>GVTELSDAQKKQLKEQQEMQQMYDMIMQHKRAMQDMQLLWEKAVQQHQHGYDSDEEVDSELGTWEHQLRRMEMDKTREWAEQLTKMGRGKHFIGDFLPPDELEKFMETFKALKEGREPDYSEYKEFKLTVENIGYQMLMKM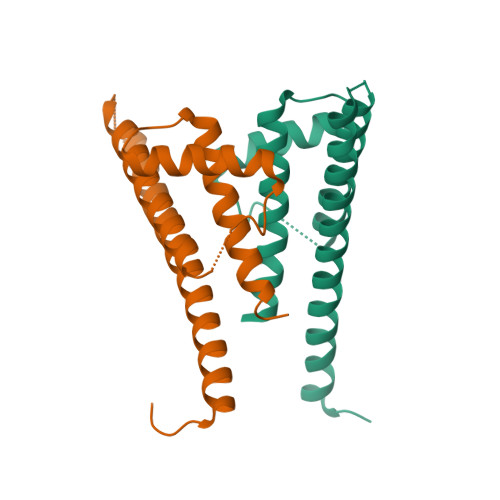GWKEGEGLGSEGQ[2x]> GPEFEAAACKKYMSKLRTIVAAQSRFLSTYDGAENLCLEDIYTENTLEVRTEVGMAGPLHKSPAALGLEELFSPNGHLNEDADTVLVVGEAGSGKSTLLQQVHLLWATGQDFQEFLFVFPFSCRQLQCVARPLSVMTLLFEHCCWPDVGQQDVFQFLLDHPDRILLTFDGFDEFKFKFTDHERHCSPTDPTSVQTLLFNLLQGNLLKNARKVLTSRPDAVSAFLRKYVRTEFNLKGFSEEGIELYLRKCHREPGVADRLIHLLQTTSALHGLCHLPVFSWMVSKCHQELLLQDGGSPKTTTDMYLLILQHFLRHASLPDSASQGLGPSLLQGRLPTLLRLGQLALWGLGMCCYVFSAQQLQAAQVDPDDISLGFLVQAQGVVPGSTAPLEFLHITFQCFLAAFYLVLSTDVPTASLRYLFNCRRPGSSPLSRLLPRLCVQGSEHKESTVAALLQKTEPHNLQITAAFLAGLLSREHRDLLAACQASERSLLRRRACARWCLARSLHKHFRSIPPAVPGEAKSMHAMPGFLWLIRSLYEMQEERLAQEAVRGLNVEHLKLTFCGVGPAECAALAFVLRHLRRPVALQLDHNSVGDIGVEQLLPCLGACKALYLRDNNISDRGICKLIEHALHCEQLQKLALFNNKLTDGCAHSVAQLLACKQNFLALRLGNNHITAEGAQVLAEGLRDNSSLQFLGFWGNKVGDKGAQALAEALSDHQSLKWLSLVGNNIGSVGAQALASMLEKNVALEELCLAANHLQDAGVCSLAEGLKRNSSLKVLKLSNNCI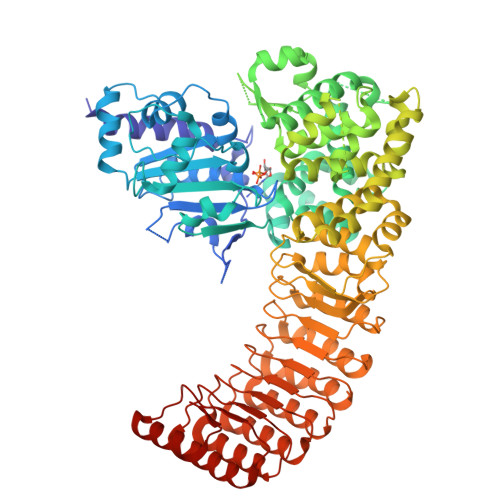TFVGAEALLQALASNDTILEVWLRGNPFSPEEMEALSHRDSRLLL> HLPPGPRPLPLLGNLLQMDRGGFLNSFRRIREKYGDVFTVHLGPRPVVMLYGTEAIREALVDQAEAFSGRGTIAVVEPIFRGYGVVFANGERWKALRRFSLVTMRDFGMGKRSVEERIQEEARCLVEEFRKSQGAPLDPTFLFQCITANIICSIVFGERFDYKDHQFLRLLYLFYQSFSLISSFSSQVFELFSGFLKYFPGTHRQISRNLQEILDYIGQSVEKHRATLDPSHPRDFIDTYLLRMEK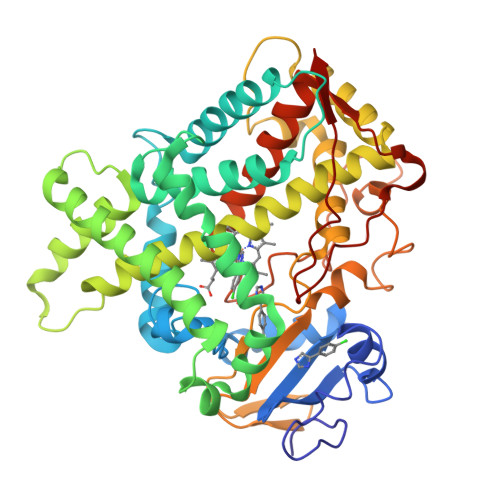EKSNQHTEFDHQNLVISVLSLFFAGTETSSTTLRYGFLLMLKYPHVAEKVQKEIDQVIGSHRLPTLEDRTKMPYTEAVIYEIQRFSDLIPIGVPHKVTKDTLFRGYLLPKNTEVYPILSSALHDPQYFEQPDTFNPDHFLDANGALKKSEAFMPFSIGKRICLGEGIARNELFLFFTTILQNFSLSSPVAPKDIDLSPKESGFGKVPQTYQICFLAR In this work, we exhaustively probe the ability of all 36 immobile HJ sequences to form DNA crystals in two different designed systems. Three separate self-assembling DNA crystal systems are described in this report: the “4 × 5” and “4 × 6” designs (collectively referred to as the 4 × N systems), and a third construct with a “scrambled” sequence variant of the 4 × 6 lattices. Self-assembly was mediated by three constituent oligonucleotides: (S1) containing four sequence repeats of either 5 or 6 bases; (S2) composed of 21 bases containing complementary regions to both (S1); and (S3) which forms the second junction crossover. The HJ serves as the fundamental component at the core of each unit, and the ultimate assembly of the full lattice is facilitated by the complementary 2-base sticky ends that tail each duplex.

We hypothesized that it might be possible to introduce other unique immobile sequences that could provide slight perturbations in the junction angle, to potentially reduce the strain in the original system and yield a “relaxed,” periodic lattice. The 4 × 5 system robustly crystallized with 75% of the junctions, and we obtained crystals in all but 9 of 36 sequences. Of the resulting structures, 18 exhibited P32 symmetry with average cell dimensions a = b = 68.85 Å c = 60.09 Å, with only nine retaining the original P3221 symmetry with average cell edges a = b = 68.17 Å c = 60.60 Å. Although the cell parameters between the two symmetries were virtually indistinguishable, the differences between the periodicity of the lattices is dramatic, with vastly different cavity sizes. We hypothesize that even a small difference in junction angles could have a significant global effect on the assembly of the lattice, thereby eliminating the strain in the P3221 lattices. However, in the majority of the crystal structures reported here, the cacodylate anion indeed fits best into the electron density map of our X-ray structures, due to the presence of sodium cacodylate in the crystallization solution.

> GAGCAGACGTG;> ACAGCACTCA;> CATGT;> TCTGAGTGCCGTCTGC> MTEIYEQAKHSLQGEDFSSFNYLFAVNKLLSNPVSYDLGRDLIVRALDSRERFSEHTTILKNMVRKSGLFPYLKKEFTSLTPDDLRVLELYRTPFSDGYVFHSMQFHIFDLLKSGQNVVLSAPTSMGKSAIVDSLLGMGTLKRLVLVVPTVALADETRRRLQERFGDRYQIIHHSSQVCHSDQAVYVLTQERVNERDDIVDIDLFVIDEFYKLAFRQLKSGDIDHQDERVIELNIALSKLLKVSRQFYLTGPFVNSIRGLEKLGYPHTFVSTDFNTVALDVKTFGIKANDDKAKLKALGEIAHACVDATIIYCKSPTVAGLVARELIRLGHGTPTENPHVDWVSEEFDADWDYTVALRNGIGLHFGALPRALQQYTADQFNAGKLRFLLCTSTIIEGVNTIAKNVVIYDNRDGTRSIDKFTHGNIKGRAGRMGVHFVGKIFCLEEIPEDNLNQEVDIPLGIQGIDTPINLLASVQPDHLSEFSQDRFDEVFINDRVSIDLVKKHSYFRVEQFEMLQSMFEMMDDNEFSSLVFHWTPATNFLKTFAKIIARLVPHTFSRNGVPVKPTDVMIAKLAGYLSAESYSEYLKNQIDYARQWISEGEKRTLSIALNNDLKLITNTFGYTLPKVLSLMEDVVKHHAVKRGIRSKVDYTHVK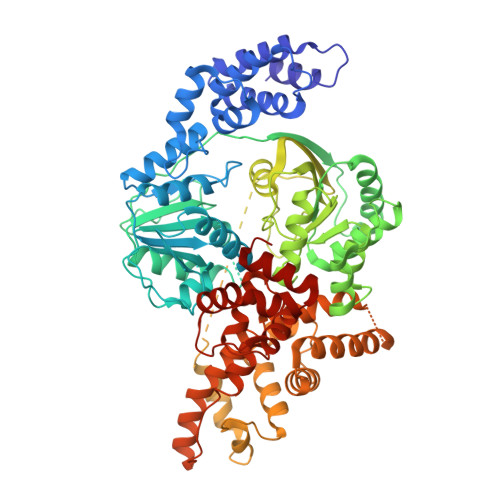LAFESFHLPPGVNALEEIGIPIQTLHRLVDLLEFSDEADVDELSQYLRDTQDIWSRSIGYVDQMFIRRALGIRRH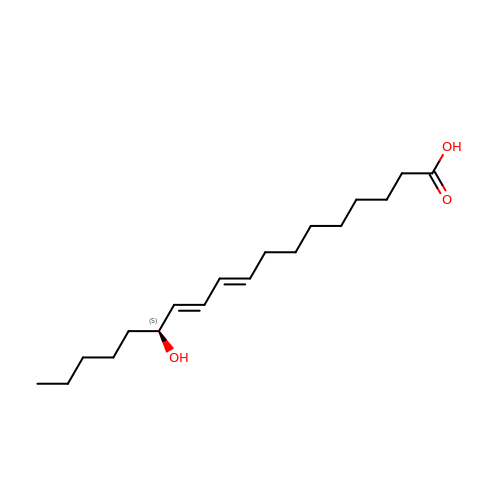(9E,11E,13S)-13-hydroxyoctadeca-9,11-dienoic acid | C18 H32 O3 | HNICUWMFWZBIFP-WHLLTAFYSA-N> GSGGSGGITEAQARAIVNSALKLYSQDKTGMVDFA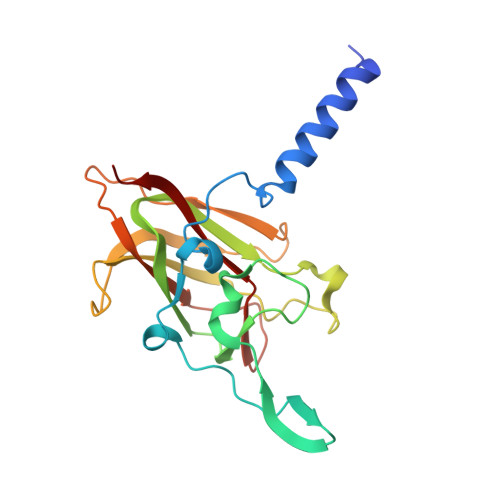LESGGGSILSTRCSETYETKTALMSLFGIPLWYFSQSPRVVIQPDIYPGNCWAFKGSQGYLVVRLSMMIHPAAFTLEHIPKTLSPTGNISSAPKDFAVYGLENEYQEEGQLLGQFTYDQDGESLQMFQALKRPDDTAFQIVELRIFSNWGHPEYTCLYRFRVHGEPVK> MKNSPLNGLNGLKAFLETKPKEYHKFDPSRFIQIYKDFKNAFFEIQAKVIHVVGTNGKGSTGRFLTLLLADQNFKVLHFTSPHVFEFRERFFLNGSVVGESVLENAHQQLQSHAFSSACSYFEYATLLAVMLAKDCDYLVLEAGLGGEFDSTNALKKTLSVFTPIDYDHKEFLGDSLESIAQTKLKAMGSLSIIAPQQELVLNAAQKIAKEKHAKLIVVQNEISKGVRDYIERYHLARFLAMNLEVALKAFETLLPCNKQEVLKNLKPLNLIGRCELLSPNILIDVGHNPHSAKALKEEIKRIFNAKIILIYNCYQDKDAFLVLEILKPVIKKVL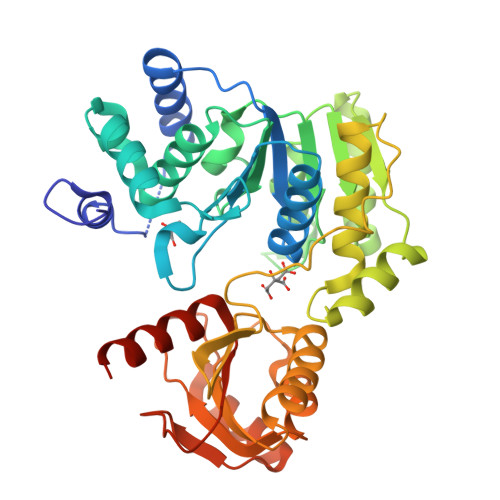ILELHEERVIKLEKLKGILETLGLEYALFEDVEENENYLVYGSFLVANAFYKRYQEKRDLEHHHHHH VmoLac (YP_004245953) is a recently identified enzyme that was isolated from the hyperthermophilic crenarchaeon Vulcanisaeta moutnovskia strain 768-2833. The phylogenetic tree that was built from this sequence alignment, indicates that VmoLac belongs to the clade of the PLLs-A. Kinetic characterization indicates that VmoLac is a proficient lactonase with promiscuous, poor esterase and phosphotriesterase activities. As expected, VmoLac is roughly globular and exhibits a (β/α)8 barrel topology that is similar to that of others PLLs such as SsoPox17, SisLac8, DrOPH3, GsP10 and GkL36.

Interestingly, VmoLac was crystallized in two different space groups. The other structure, solved in P622, contains only one protein molecule in the asymmetric unit. The dimer can be reconstructed by symmetry, and the observation of the other neighboring molecules reveals another, weaker interaction within the crystal packing. The contacting surface in this interaction is much smaller (616 Å2) and involves 4 hydrogen bonds and 4 salt bridges. Intriguingly, this contact mode between the two protein molecules connects the two active sites hydrophobic channels. As expected, both of the structures are nearly identical (r.m.s.d for α-carbon atoms (over 315 atoms) of 0.34 Å), but some slight differences can be observed in the active site region (loops 7 and 8). A clear extra density was observed in the active sites of both of the VmoLac structures, although no potential substrates were present in the crystallization conditions. Because of a relatively good resolution of the structures (1.8 and 2.35 Å), this unexpected density could be attributed to a fatty acid with good confidence. Therefore, this density was attributed to the simplest fatty acid that fit the observed density and that was present in the expression host E. coli: myristic acid. The carboxylate of the fatty acid molecule is tightly bound to the bi-metallic active site (2.2 Åα–2.3 Åβ), while the long aliphatic fatty chain that sits in the hydrophobic channel is mainly formed by loop 8 residues.

> GMVRISIAGGNEIDPGSMGLTLFHEHLRLITEVVRWNWPHLYNEDEELKRAIDAVNAAKKYGVKTIIDLTVAGIGCDVRFNEKVAKATGVNIIMGTGFYTYTEIPFYFKNRGIDSLVDAFVHDITIGIQGTNTRAAFVKAVIDSSGLTKDVEMAIRAAAKAHIKTDVPIITHSFVGNKSSLDLIRIFKEEGVDLARTVIGHVGDTDDISFIEQILREGAFIGLDRFGLDIYLPLDKRVKTAIELIKRGWIDQLLLSHDYCPTIDWYPPEVVRSTVPDWTMTLIFEKVIPRMRSEGITEEQINRVLIDNPRRLFTGR>[2x]MDDLDLPDPSLKNIIDQTTLQWVFVGGKGGVGKTTTSCCLGVQLAKSRTKVLLVSTDPAHNLSDAFCQKIGREPTPIHGFDNLCAMEIDASQEAESEIEATDDNDVFGQMFNDLQNSIPGIDEAMSFSELMKQVQQLDFDVVVFDTAPTGHTLRLLSFPTILEKAFAKVWELKDRFGGLIGQATALMSGGNNPAAAQEQLLGKLEETRAVINKVNQAFQDPTKTTFVCVCIPEFLSIYETERLVQELSKYGIDSHNIVVNQVLFPEKDAEELSAWYEANGATLPKEAREICSKLLARKRMQDKYIGQCFDLYGDDFHVVLMPLLDYEVRGVEKLKTFSELLVDPVDMDE

A functionally diverse set of tail-anchored (TA) membrane proteins are delivered and inserted into the ER through a posttranslational pathway, termed the guided entry of TA protein (GET) system. In eukaryotes, ranging from microbes to animals, the GET system is mediated by a cytosolic ATPase (termed as TRC40 or ASNA-1 in humans and Get3 in fungi), which coordinates the translocation of TA proteins to the ER by binding with ER-bound receptors (WRB/CAML in mammals, Get1/2 in yeast and Arabidopsis). In this study, we identified two isoforms of Get3 in Phaeodactylum tricornutum, a cytosolic Pt-Get3a and a chloroplast-localized Pt-Get3b protein. Furthermore, we solved the crystal structure of Pt-Get3a and determined that it does not contain the conserved CXXC motif, potentially leading to the spontaneous formation of a distinct parallelogram-shaped dimer in solution.

Moreover, we observed the apo-form crystal of Pt-Get3a at a resolution of 3.8 Å in the space group as I212121. Two molecules of Pt-Get3a in one asymmetric unit formed a homodimer in both apo and nucleotide-bound Pt-Get3a structures. However, both the structures were similar, with their RMSD ranging from 0.47 to 0.87 Å over all backbone Cα atoms. Moreover, Pt-Get3a existed as a distinct parallelogram-shaped dimer in the crystal, which markedly differed from the structures of classic U-shaped Get3 dimers. The parallelogram-shaped dimer might form due to the lack of the zinc-bound CXXC motif, which coordinates the open-to-closed transition of Get3 for TA protein targeting. In addition, an ellipsoid-shaped tetramer of Pt-Get3a was observed through crystal packing in both crystal structures. Two parallelogram-shaped dimers (A/B and C/D) were assembled in a crystallographic tetramer aligned along the long axis of symmetry. The ellipsoid-shaped tetramer of Pt-Get3a could alternatively consist of two crystallographic homodimers of A/D and B/C monomers aligned along the short axis of symmetry, similar to the classic U-shaped formation of Get3 in the dimer state. Because of the lack of the conserved CXXC motif, monomers in a U-shaped Pt-Get3a dimer (A/D or B/C) are associated through two α-helical hairpins (α10 and N terminus of α11) from each monomer, which are located at the equivalent area of the CXXC motif in other Get3 crystal structures.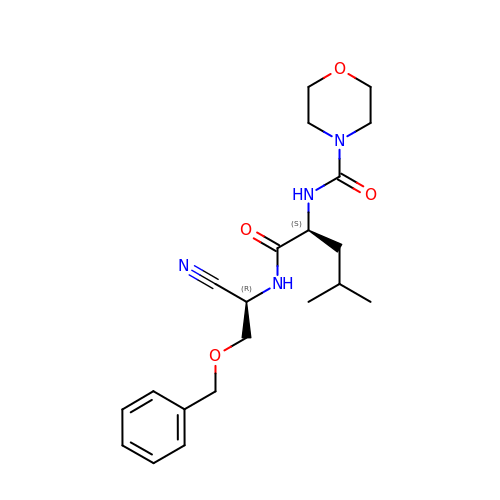MORPHOLINE-4-CARBOXYLIC ACID [1S-(2-BENZYLOXY-1R-CYANO-ETHYLCARBAMOYL)-3-METHYL-BUTYL]AMIDE | C21 H30 N4 O4 | LXEDKIMJQBOMSU-MOPGFXCFSA-N> VILPNNNRHQIFNTTQGHYDAVSFIYIPIDGGYMSGSGVVVGENEILTNKHVVNGAKGNPRNISVHPSAKNENDYPNGKFVGQEIIPYPGNSDLAILRVSPNEHNQHIGQVVKPATISSNTDTRINENITVTGYPGDKPLATMWESVGKVVYIGGEELRY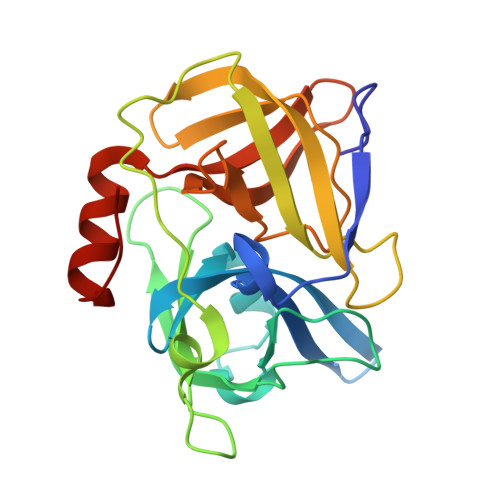DLSTVGGNSGSPVFNGKNQVIGIHYGGVDNKYNSSVYINDFVQQFLRNNIPDINIQ>SEPLVRFKRSVNITKGDLNSWRTGTDPCNGKWFGIYCQKGQTVSGIHVTRLGLSGTINIEDLKDLPNLRTIRLDNNLLSGPLPPFFKLPGLKSLLLSNNSFSGEIADDFFKETPQLKRVFLDNNRLSGKIPASLMQLAGLEELHMQG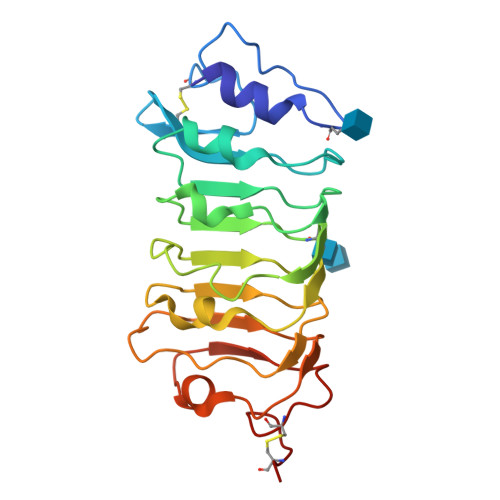NQFTGEIPPLTDGNKVLKSLDLSNNDLEGEIPITISDRKNLEMKFEGNQRLCGSPLNIECD[2x]> SGDYRVQNTSLEAIVQNASSDNQGIQLSAVQAARKLLSSDRNPPIDDLIKSGILPILVHCLERDDNPSLQFEAAWALTNIASGTSEQTQAVVQSNAVPLFLRLLHSPHQNVCEQAVWALGNIIGDGPQCRDYVISLGVVKPLLSFISPSIPITFLRNVTWVMVNLCRHKDPPPPMETIQEILPALCVLIHHTDVNILVDTVWALSYLTDAGNEQIQMVIDSGIVPHLVPLLSHQEVKVQTAALRAVGNIVTGTDEQTQVVLNCDALSHFPALLTHPKEKINKEAVWFLSNITAGNQQQVQAVIDANLVPMIIHLLDKGDFGTQKEAAWAISNLTISGRKDQVAYLIQQNVIPPFCNLLTVKDAQVVQVVLDGLSNILKMAEDEAETIGNLIEECGGLEKIEQLQNHENEDIYKLAYEIIDQFFSSDDIDEDPSLVPEAIQGGTFGFNSSANVPTEGFQF;> RKARKRSHSPTKKLRYVKRRF

The MERS-CoV ORF4b protein is a viral accessory protein that functions as an innate immune inhibitor and strongly localizes to the nucleus, despite virus replication occurring exclusively within the cytoplasmic compartment. The MERS-CoV ORF4b protein has been shown to bind preferentially to the nuclear import adapter IMPα3 in infected cells, thereby inhibiting NF-κB-dependent innate immune responses. Here we provide a detailed, structural basis for the interaction between MERS-CoV ORF4b and its innate immune suppression target, the nuclear import adapter IMPα. Our results provide a detailed structural basis that explains how a virus can target the IMPα nuclear import adapter to impair immunity, and illustrate how small mutations in ORF4b, like those found in closely related coronaviruses such as HKU5, change the IMPα binding mechanism.

Because the results indicated that MERS-CoV ORF4b NLS was able to bind IMPα isoforms with high affinity and showed little preference for a specific isoform, we examined the molecular interface with two IMPα isoforms using high-resolution structural approaches. Specifically, we crystallized the MERS-CoV ORF4b NLS bound to both IMPα2 and IMPα3 and resolved the structures to 2.1 Å and 2.5 Å resolution respectively (see Supplementary Table 1 for data collection and refinement statistics). F Crystal structure of MERS-CoV ORF4b NLS bound to IMPα3 at 2.5 Å resolution. Our high-resolution crystal structures showed that MERS-CoV ORF4b occupies an extensive interface across both IMPα2 and IMPα3. Strikingly, the binding interface of both structures lacked a Lys at the P2 position within the major site that is seen with other NLSs. Surprisingly, MERS ORF4b does not contain a Lys at the P2 site, but rather a Val (position 35), which did not form any interactions with the Gly150, Thr155, and Asp192 pocket. Rather, MERS ORF4b bound IMPα2 and IMPα3 through an Arg residue (position 33, the equivalent of the P0 position) at this site and formed similar interactions to those made by a Lys NZ nitrogen at the P2 site. Paradoxically, this interaction interface was very similar in both the nuclear import adapter IMPα2 and in IMPα3, the latter of which ORF4b reportedly exhibited a binding preference.> CEVPTRLNSASLKQPYITQNYFPVGTVVEYECRPGYRREPSLSPKLTCLQNLKWSTAVEFCKKKSCPNPGEIRNGQIDVPGGIL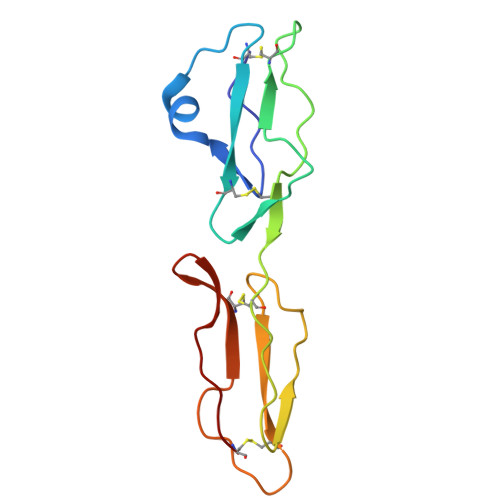FGATISFSCNTGYKLFGSTSSFCLISGSSVQWSDPLPEC>[4x]GPLGSPEFQKTKPFSVPNLPLNTLSNSRVPSLIRSMMVSRDHGQMVQFQNGRVTLDGQLQGTTPTSASQLCKIRGSVFHANGGNGYNLTELDGSPYHAFESPAPIGFPDLGECDWHMEASPTTQFDTGDVIKQINVKQEAAFAPHLGTIQADGLS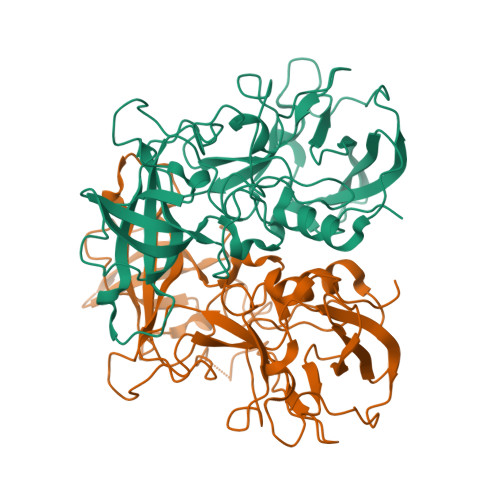DVSVNTNMIAKLGWVSPASDGHRGNVDPWVIPRYGSTLTEAAQLAPPIYPPGFGEAIVFFMSDFPIAHGANGLSVPCTIPQEFVTHFVNEQAPTRGEAALLHYLDPDTHRNLGEFKLYPEGFMTCVPNSSGTGPQTLPINGVFVFVSWVSRFYQLKPVGTAGPARSLGIRRS>[8x]MEPHDTLSPAQVDEYRKNGFLVQEHVFDEEEIELLRAEAAQEFASGGERVTVEQNTGIVRGVHGCHLYSEVFGRLVRSPRLLPIARQLLRDDVYVHQFKIIAKRAFKGEVWEWHQDYTFWHHEDGMPAPRALSAAIFLDEVTEFNGPLTFVPGGHGSGMIDADVKGEGWANTLTASLKYSLDVETMRGLIERNGMVAPKGPRGSVLWFDANIP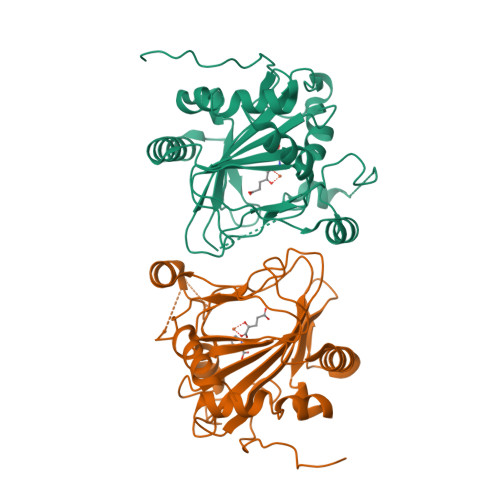HSSVPNISPFDRGLVLITYNSVENKTDVTRGTRPEWLAARDFTPLTALQATSF>[2x]MSMAMSQSNRELVVDFLSYKLSQKGYSWSQFSDVEENRTEAPEGTESEAVKQALREAGDEFELRYRRAFSDLTSQLHITPGTAYQSFEQVVNELFRDGVNWGRIVAFFSFGGALC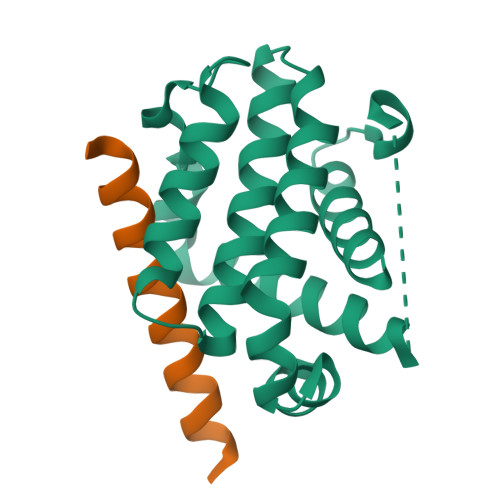VESVDKEMQVLVSRIAAWMATYLNDHLEPWIQENGGWDTFVELYGNNAAAESRKGQERLEHHHHHH;> DPVPQDASTKKLSECLKRIGDELDSNMELQRMIA> GMMNKPAPRELEVIRSTYITPHMLRITLGGAGLAGFPADQESAYIKLLFPQAGERPLMRTYTIRQQRDDEIDVDFVLHDTDGPASSWAKTAQVGELIQIGGPGLKKLINFEADWFLLAGDMTALPAISVNLA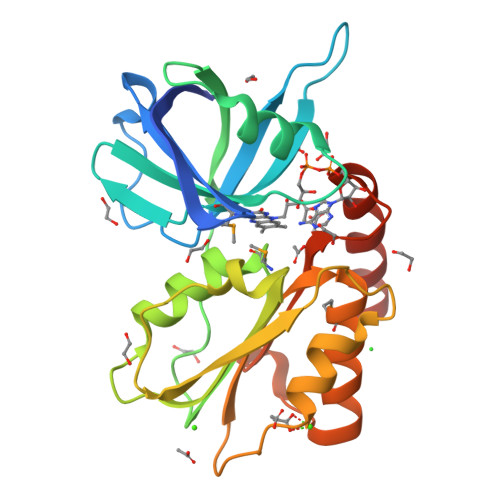KLPNNAVGYAVIEVLSEADIQPLVHPEHVELHWVINPEADPEGRPLVERIAQLPWLAGEPAVWIACEFNSMRALRRHFKQAHALPKSHFYTSSYWKIGCNEGEHKLVKQEDEQLENGASV> LYFSRDAYWEKLYVDQAAGTPLLYVHALRDAPEEVPSFRLGQHLYGTYRTRLHENNWICIQEDTGLLYLNRSLDHSSWEKLSVRNHGFPLLTVYLKVFLSPTSLREGECQWPGCARVYFSFFNTSFPACSSLKPRELCFPETRPSFRIRENRPPGTFHQFRLLPVQFLCPNISVAYRLLEGEGLPFRCAPDSLEVSTRWALDR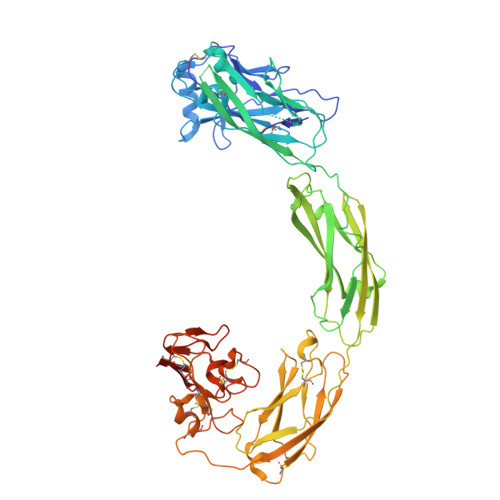EQREKYELVAVCTVHAGAREEVVMVPFPVTVYDEDDSAPTFPAGVDTASAVVEFKRKEDTVVATLRVFDADVVPASGELVRRYTSTLLPGDTWAQQTFRVEHWPNETSVQANGSFVRATVHDYRLVLNRNLSISENRTMQLAVLVNDSDFQGPGAGVLLLHFNVSVLPVSLHLPSTYSLSVSRRARRFAQIGKVCVENCQAFSGINVQYKLHSSGANCSTLGVVTSAEDTSGILFVNDTKALRRPKCAELHYMVVATDQQTSRQAQAQLLVTVEGSYVAEEAGCPLSCAVSKRRLECEECGGLGSPTGRCEWRQGDGKGITRNFSTCSPSTKTCPDGHCDVVETQDINICPQDCLRGSIVGGHEPGEPRGIKAGYGTCNCFPEEEKCFCEPEDIQDPLCDELCRGTHHHHHHHH>GSASLTEIEHLVQSVCKSYRETCQLRLEDLLRQRSNIFSREEVTGYQRKSMWEMWERCAHHLTEAIQYVVEFAKRLSGFMELCQNDQIVLLKAGAMEVVLVRMCRAYNADNRTVFFEGKYGGMELFRALGCSELISSIFDFSHSLSALHFSEDEIA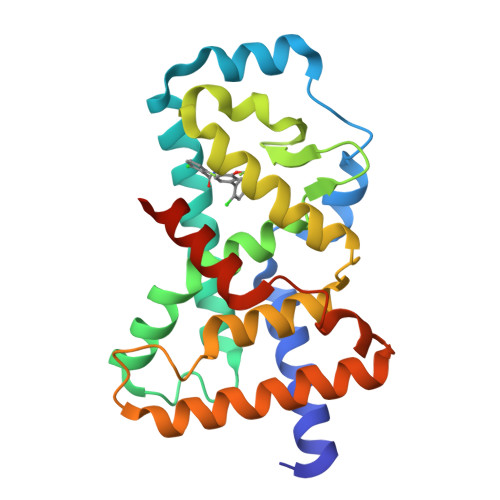LYTALVLINAHRPGLQEKRKVEQLQYNLELAFHHHLCKTHRQSILAKLPPKGKLRSLCSQHVERLQIFQ[4x]>[2x]SMSKNNIFNKYPTIIHGEARGENDEFVVHTRYPRFLARKSFDDNFTGEMPAKPVNGELGQIGEPRRLAYDSRLGLWLSDFIMLDNNKPKNMEDWLGQLKAACDRIAADDLMLNEDAADLEGWDD;> SMAAFKPNSINYILGLDIGIASVGWAMVEIDEEENPIRLIDLGVRVFERAEVPKTGDSLAMARRLARSVRRLTRRRAH

In this work, we investigate the mechanism of activity of anti-CRISPR protein AcrIIC2Nme. This 123-residue protein was previously shown to inhibit the activity of Neisseria meningitidis CRISPR-Cas9 in vivo and in vitro. We show that AcrIIC2Nme functions by inhibiting loading of the guide RNA molecule, thereby preventing formation of the active CRISPR-Cas9 surveillance complex. We found that it blocks Cas9 binding to sgRNA, thereby inhibiting biogenesis of the surveillance complex. This interference is mediated through an interaction with the arginine-rich bridge helix, which connects the REC lobe to the NUC lobe.

We also solved the crystal structure of AcrIIC2Nme in complex with Nme1Cas9 to a resolution of 2.6 Å. We found that AcrIIC2Nme bound to Nme1Cas9 in the same dimeric form as observed in the unbound state. Unexpectedly, only residues 16–77 of Nme1Cas9, corresponding to the bridge helix region and a partial fragment I of the RuvC domain, were observed in the complex. Analysis of the AcrIIC2-Nme1Cas9 crystal by SDS-PAGE revealed that the rest of Nme1Cas9 was digested during crystallization. The AcrIIC2Nme monomers form a dimer with a negatively charged surface on one side into which the arginine-rich bridge helix nestles. Four residues from each of the AcrIIC2Nme monomers, E17, E24, D108, and N112, make interactions with the bridge helix. In AcrIIC2.1, the side-chain of E17 hydrogen bonds with Nme1Cas9 residues R69 and R73, E24 interacts with residues R73 and R74, while D108 and N112 form hydrogen bonds with the side-chain of R74. Similarly, the side-chains of E24, D108, E17, and N112 of AcrIIC2.2 interact with Nme1Cas9 residues R62, R66, R69, and R70. To further establish the impact of AcrIIC2Nme binding on the assembly of Nme1Cas9 with sgRNA, we compared the structure of AcrIIC2Nme bound to Nme1Cas9 with the Nme1Cas9-sgRNA binary complex by aligning the bridge helix regions. The structural superposition shows that two AcrIIC2Nme monomers make major clashes with stem loops 1 and 2, and slightly overlap the seed region of the sgRNA.>[4x]MSVNNPQTREWQTLSGEHHLAPFSDYKQLKEKGPRIITKAQGVHLWDSEGHKILDGMAG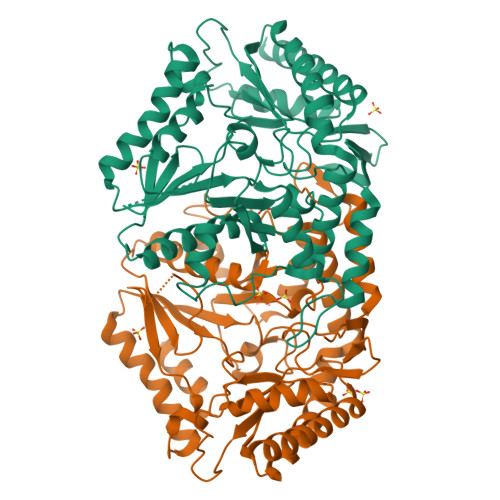LWCVAVGYGREELVQAAEKQMRELPYYNLFFQTAHPPALELAKAITDVAPKGMTHVFFTGSGSEGNDTVLRMVRHYWALKGKPHKQTIIGRINGYHGSTFAGACLGGMSGMHEQGGLPIPGIVHIPQPYWFGEGGDMTPDEFGVWAAEQLEKKILEVGEDNVAAFIAEPIQGAGGVIIPPETYWPKVKEILARYDILFVADEVICGFGRTGEWFGSDYYDLKPDLMTIAKGLTSGYIPMGGVIVRDTVAKVISEGGDFNHGFTYSGHPVAAAVGLENLRILRDEKIVEKARTEAAPYLQKRLRELQDHPLVGEVRGLGMLGAIELVKDKATRSRYEGKGVGMICRTFCFENGLIMRAVGDTMIIAPPLVISHAEIDELVEKARKCLDLTLEAIQ β1,3-N-acetylglucosaminyltransferases (B3GNTs) are Golgi-resident glycosyltransferases involved in the biosynthesis of poly-N-acetyl-lactosamine chains. They catalyze the addition of the N-acetylglucosamine to the N-acetyl-lactosamine repeat as a key step of the chain elongation process. Among the characterized B3GNTs, B3GNT2 is the major poly-N-acetyl-lactosamine synthase, and deletion of its coding gene dramatically reduced the cell surface poly-N-acetyl-lactosamine and led to hypersensitive and hyperresponsive immunocytes. The luminal domain of B3GNT2 comprises an N-terminal helical domain (Pro55–Cys125) and a C-terminal catalytic domain (Cys138–Cys397) as well as an extended linker (Arg126–Lys137) that connects the helical domain to the catalytic domain.

By soaking B3GNT2 crystals with either the donor substrate UDP-GlcNAc or the acceptor substrate LacNAc, we were able to obtain B3GNT2 structures (B3GNT2_UDPGlcNAc and B3GNT2_LacNAc) in the substrate-bound states. The acceptor substrate LacNAc (Galβ1-4GlcNAc) is bound to the top of the cleft and more solvent exposed. The Gal ring for the anticipated glycosidic bond formation reaction is located close to the center of the cleft, whereas the GlcNAc ring is close to the solvent. The hydroxyls of the Gal ring are engaged in direct hydrogen bond interactions with the side chains of His282 and Asp333 and water-mediated hydrogen bond interaction with the side chain of Tyr300. The Gal ring is also stacked against the side chain of Tyr289. In contrast, the GlcNAc ring is only involved in a water-mediated hydrogen bond with the main chain oxygen of Gly280 through one of its hydroxyls. And superposition of the B3GNT2_UDPGlcNAc and B3GNT2_LacNAc structures shows that the acceptor substrate LacNAc binds right above the donor substrate UDP-GlcNAc in the substrate-binding cleft. The hydroxyl group on C3 of the Gal in the acceptor substrate points to the C1 of the GlcNAc in the donor substrate at a distance of 3.7 Å. The Asp333, which is 2.7 Å from the hydroxyl group on C3 of Gal in the acceptor substrate LacNAc, serves as the active site base and abstracts the proton from this hydroxyl group. Ala279 from the β5-β6 loop is less than 4 Å from the acetyl group of the GlcNAc of the acceptor substrate.

>MHHHHHHHHENLYFQGSKEKFWKISTPPEAYWNREQEKLNRQYNPILSMLTNQTGEAGRLSNISHLNYCEPDLRVTSVVTGFNNLPDRFKDFLLYLRCRNYSLLIDQPDKCAKKPFLLLAIKSLTPHFARRQAIRESWGQESNAGNQTVVRVFLLGQTPPEDNHPDLSDMLKFESEKHQDILMWNYRDTFFNLSLKEVLFLRWVSTSCPDTEFVFKGDDDVFVNTHHILNYLNSLSKTKAKDLFIGDVIHNAGPHRDKKLKYYIPEVVYSGLYPPYAGGGGFLYSGHLALRLYHITDQVHLYPIDDVYTGMCLQKLGLVPEKHKGFRTFDIEEKNKNNICSYVDLMLVHSRKPQEMIDIWSQLQSAHLKC[2x]>GMEPFKQQKVEDFYDIGEELGSGQFAIVKKCREKSTGLEYAAKFIKKRQSRASRRGVSREEIEREVSILRQVLHHNVITLHDVYENRTDVVLILELVSGGELFDFLAQKESLSEEEATSFIKQILDGVNYLHTKKIAHFDLKPENIMLLDKNIPIPHIKLIDFGLAHEIEDGVEFKNIFGTPEFVAPEIVNYEPLGLEADMWSIGVITYILLSGASPFLGDTKQETLANITSVSYDFDEEFFSHTSELAKDFIRKLLVKETRKRLTIQEALRH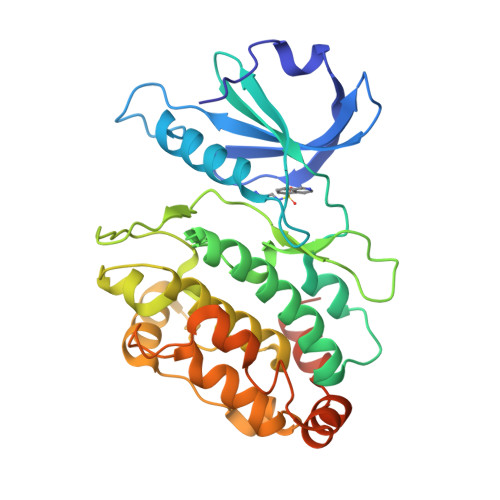PWITPVDNQQAMVRRESVVNLENFRKQYVRRRWKLSFSIVSLCNHLTR[4x]>GSHMASMGVTVQDICFAFLQNYYERMRTDPSKLAYFYASTAELTHTNYQSKSTNEKDDVLPTVKVTGRENINKFFSRNDAKVRSLKLKLDTIDFQYTGHLHKSILIMATGEMFWTGTPVYKFCQTFILLPSSNGSTFDITNDIIRFISNSFKLE[2x];>GSASVTKLKNLKENSSNLIQLPLFINTTEAEFAAASVQRYELNM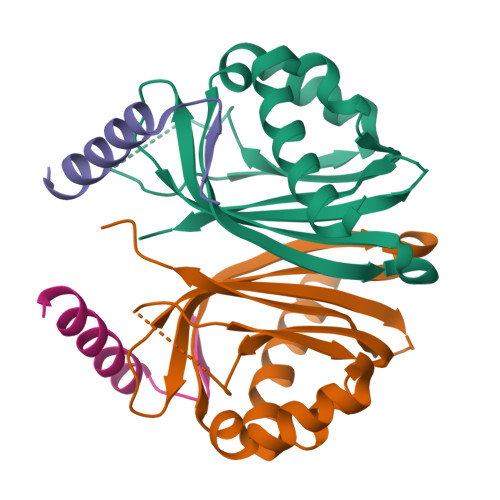KALN[2x]>[2x]MSGSHHHHHHSG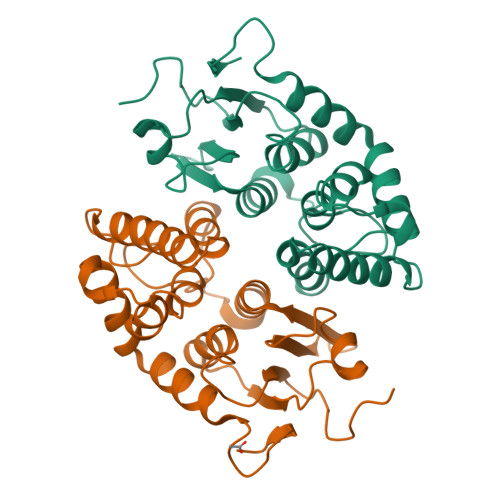SMSERPSDLVVNRLVLFVVKGTATSTHNTVKPLILLEELGVPHDIYVVEKVSAPWFSEINPHKMVPAILDRSPDGRDTLRAWESTSTLMYIADAYDKDGTFGGRNVQERSEINNWLTLHTAALGPTAKYWLYFYKLHPEKLPKTIEKLRSNITVQYDILERRLNEPGQQYLALKDRPTIADIATLPFAMKSTAELFGLEFEKWPKLQEWSVRMGEREAVKRAWQRVAGFGHGEKEYGMLEA> MSTQYETQGYTINNAGRRLVVDPITRIQGHMRCEVNINDQNVITNAVSCGTMFRGLEIILQGRDPRDAWAFVERICGVCTGVHALASVYAIEDAIGIKVPDNANIIRNIMLATLWCHDHLVHFYQLAGMDWIDVLDALKADPRKTSELAQSLSSWPKSSPGYFFDVQNRLKKFVEGGQLGIFRNGYWGHPQYKLPPEANLMGFAHYLEALDFQREIVKIHAVFGGKNPHPNWIVGGMPCAINIDESGAVGAVNMERLNLVQSIITRTADFINNVMIP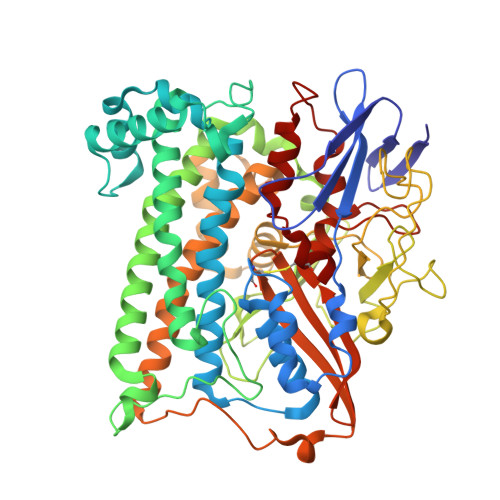DALAIGQFNKPWSEIGTGLSDKCVLSYGAFPDIANDFGEKSLLMPGGAVINGDFNNVLPVDLVDPQQVQEFVDHAWYRYPNDQVGRHPFDGITDPWYNPGDVKGSDTNIQQLNEQERYSWIKAPRWRGNAMEVGPLARTLIAYHKGDAATVESVDRMMSALNLPLSGIQSTLGRILCRAHEAQWAAGKLQYFFDKLMTNLKNGNLATASTEKWEPATWPTECRGVGFTEAPRGALGHWAAIRDGKIDLYQCVVPTTWNASPRDPKGQIGAYEAALMNTKMAIPEQPLEILRTLHSFDPCLACSTH>SPTNLAKVKGITQGPNESPSAFLERLKEAYRRYTPYDPEDPGQETNVSMSFIWQSAPDIGRKLERLEDLKSKTLGDLVREA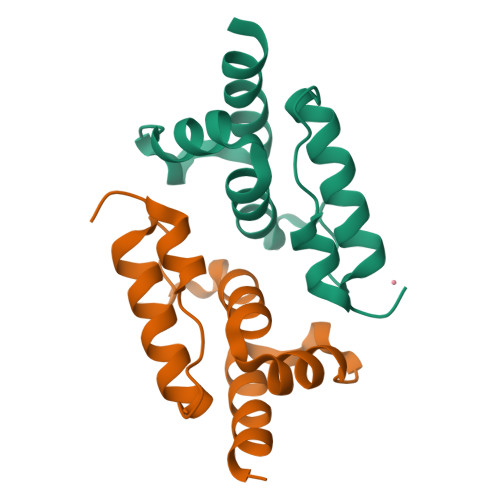EKIFNK[2x]>[2x]MGSSHHHHHHSSGLVPR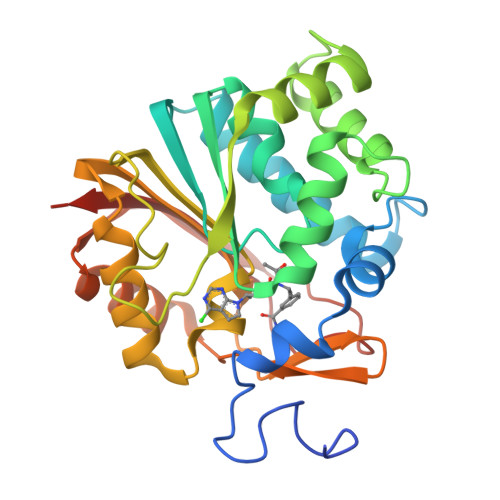GSMESGFTSKDTYLSHFNPRDYLEKYYKFGSRHSAESQILKHLLKNLFKIFCLDGVKGDLLIDIGSGPTIYQLLSACESFKEIVVTDYSDQNLQELEKWLKAAPAAFDWSPVVTYVCDLEGNRVKGPEKEEKLRQAVKQVLKCDVTQSQPLGAVPLPPADCVLSTLCLDAACPDLPTYCRALRNLGSLLKPGGFLVIMDALKSSYYMIGEQKFSSLPLGREAVEAAVKEAGYTIEWFEVISQSYSSTMANNEGLFSLVARKLSRPL>MRDTLVLNAFHMNTVCHMYDGGWRNPADRQVEFATLEFWKEVAQTLERGFFDSLFFADVMGTDAAYGDSWDIYAEQGIHFPMHDAASLVAALIPHTEHLGLTFSSSVIQDHPFSFAKRASTLDHLSGGRVGWNIVTGGTINASQNFGYDSLVPHDERYAIGEEYMEVVYKLWEGSWDEGALVADKTKGIYADPSKIHKINHRGERYRVAGPHLTLPSPQRTPFLFQAGASTAGRAFASRHAEATLVLCLTPDSMRVAYK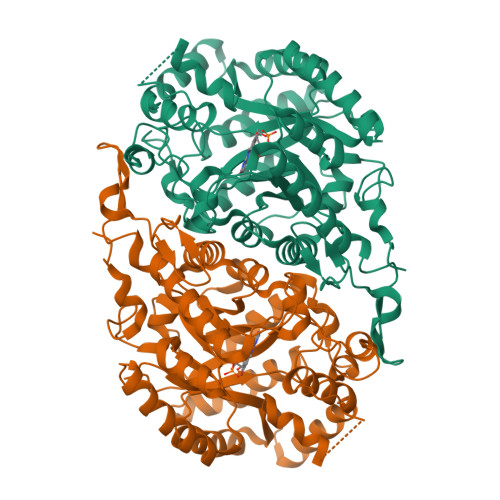QMQELLAAAGRASDDLLMVQGMSFIVGSTEEEARRKAEEQDQYLDVDALAARVSRDLGVDLSGADADQPLDTIQTEATQGIAKLMMEAVPDGRPKVKDLPLLYSIRIVGTPETIADELTEWRDAGMGGINMAAQMLPGTDADFVDYVVPELQRRGMVQHEYRPGTLREKVFPGRDRLLNERHPASRYRGIFS[2x]>[3x]M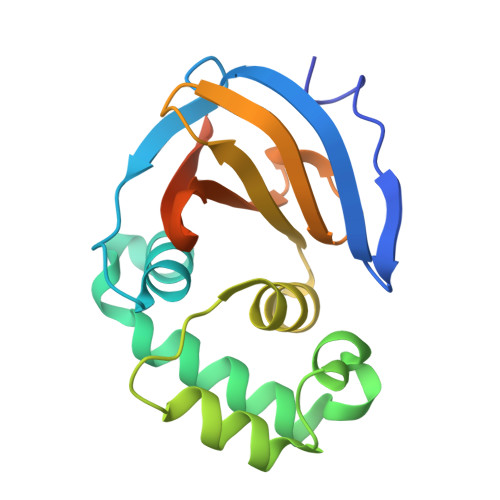ANLKENIVWEHVFDNCSQANVVFSYREFFNKELTLPDGNCFFRAVSTFLYDTQNGWIEVKNMCREFAETNWDELPGVHQYFQDPEHYARESKREGYWGGSVEAEILSKLLKLTVIFWKCEDDVWVTQGIRWGDGNYLTAINLLHIQFDHFDFLVPINVTQEPPKSGSHHHHHH> PISPIETVPVKLKPGMDGPKVKQWPLTEEKIKALVEICTEMEKEGKISKIGPENPYNTPVFAIKKKDSTKWRKLVDFRELNKRTQDFWEVQLGIPHPAGLKKKKSVTVLDVGDAYFSVPLDEDFRKYTAFTIPSINNETPGIRYQYNVLPQGWKGSPAIFQSSMTKILEPFKKQNPDIVICQYMDDLYVGSDLEIGQHRTKIEELRQHLLRWGLTTPDKKHQKEPPFLWMGYELHPDKWT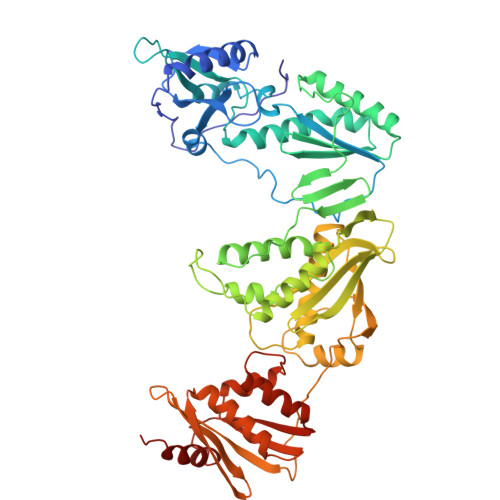VQPIVLPEKDSWTVNDIQKLVGKLNWASQIYPGIKVRQLSKLLRGTKALTEVIPLTEEAELELAENREILKEPVHGVYYDPSKDLIAEIQKQGQGQWTYQIYQEPFKNLKTGKYARMRGAHTNDVKQLTEAVQKITTESIVIWGKTPKFKLPIQKETWETWWTEYWQATWIPEWEFVNTPPLVKLWYQLEKEPIVGAETFYVDGAANRETKLGKAGYVTNKGRQKVVPLTNTTNQKTELQAIYLALQDSGLEVNIVTDSQYALGIIQAQPDKSESELVNQIIEQLIKKEKVYLAWVPAHKGIGGNEQVDKLVSAGIRK> MGEKLELRLKSPVGAEPAVYPWPLPVYDKHHDAAHEIIETIRWVCEEIPDLKLAMENYVLIDYDTKSFESMQRLCDKYNRAIDSIHQLWKGTTQPMKLNTRPSTGLLRHILQQVYNHSVTDPEKLNNYEPFSPEVYGETSFDLVAQMIDEIKMTDDDLFVDLGSGVGQVVLQVAAATNCKHHYGVEKADIPAKYAETMDREFRKWMKWYGKKHAEYTLERGDFLSEEWRERIANTSVIFVNNFAFGPEVDHQLKERFANMKEGGRIVSSKPFAPLNFRINSRNLSDIGTIMRVVELSPLKGSVSWTGKPVSYYLHTIDRTILENYFSSLKNPKLREEQEAARRRQQ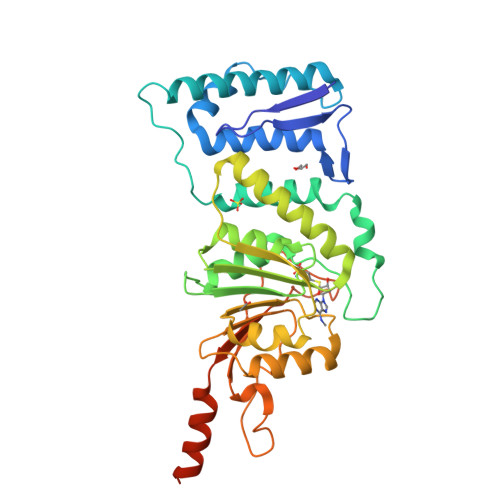RESKS>[2x]SNAPTNIHKIHEVQKKLQEEVSIVLIDIADIIVNPKKENGYSRDLYTLNSLIDSSISETYDNINNTLLSDTRFFLEH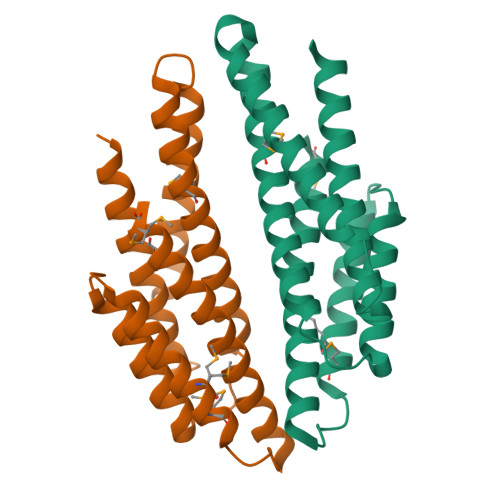MDIIKSQRDILENLYSYVSQLNSTPPQAHILSAFIHKIGYTEFEAETGNLLLEELKRLMISMKNQPLPVDRTEFENRAILFLCLTELKQFLVNRKHAQML>[7x]MAEQKSSNGGGGGGDVVINVPVEEASRRSKEMASPESEKGVPFSKSPSPEISKLVGSPNKPPRAPNQNNVGLTQRKSFARSVYSKPKSRFVDPSCPVDTSILEEEVREQLGAGFSFSRASPNNKSNRSVGSPAPVTPSKVVVEKDEDEEIYKKVKLNREMRSKISTLALIESAFFVVILSALVASLTINVLKHHTFWGLEVWKW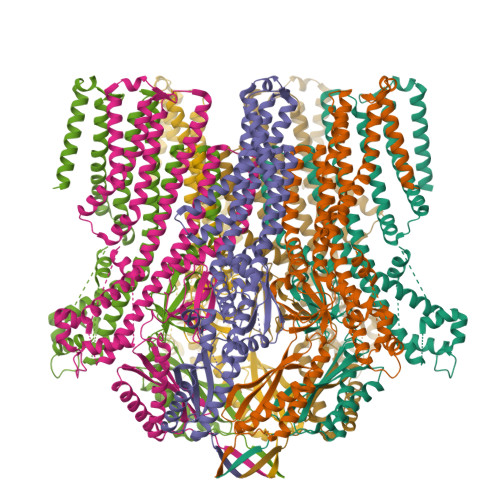CVLVMVIFSGMLVTNWFMRLIVFLIETNFLLRRKVLYFVHGLKKSVQVFIWLCLILVAWILLFNHDVKRSPAATKVLKCITRTLISILTGAFFWLVKTLLLKILAANFNVNNFFDRIQDSVFHQYVLQTLSGLPLMEEAERVGREPSTGHLSFATVVKKGTVKEKKVIDMGKVHKMKREKVSAWTMRVLMEAVRTSGLSTISDTLDETAYGEGKEQADREITSEMEALAAAYHVFRNVAQPFFNYIEEEDLLRFMIKEEVDLVFPLFDGAAETGRITRKAFTEWVVKVYTSRRALAHSLNDTKTAVKQLNKLVTAILMVVTVVIWLLLLEVATTKVLLFFSTQLVALAFIIGSTCKNLFESIVFVFVMHPYDVGDRCVVDGVAMLVEEMNLLTTVFLKLNNEKVYYPNAVLATKPISNYFRSPNMGETVEFSISFSTPVSKIAHLKERIAEYLEQNPQHWAPVHSVVVKEIENMNKLKMALYSDHTITFQENRERNLRRTELSLAIKRMLEDLHIDYTLLPQDINLTKKNSLEVLFQ> MGSHHHHHHSSGLVPRGSHMFKREEIIEMANKDFEKAWIETKDLIKAKKINESYPRIKPVFGKTHPVNDTIENLRQAYLRMGFEEYINPVIVDERDIYKQFGPEAMAVLDRCFYLAGLPRPDVGLSDEKISQIEKLGIKVSEHKESLQKILHGYKKGTLDGDDLVLEISNALEISSEMGLKILEDVFPEFKDLTAVSSKLTLRSHMTSGWFLTVSDLMNKKPLPFKLFSIDRCFRREQKEDKSHLMTYHSASCAIAGEGVDINDGKAIAEGLLSQFGFTNFKFIPDEKKSKYYTPETQTEVYAYHPKLKEWLEVATFGVYSPVALSKYGIDVPVMNLGLGVERLAMISGNFADVREMVYPQFYEHKLNDRNVASMVKLDKVPVMDEIYDLTKELIESCVKNKDLKSPCELAIEKTFSFGKTKKNVKINIFEKEEGKNLLGPSILNEIYVYDGNVIGIPESFDGVKEEFKDFLEKGKSEGVATGIRYIDALCFKITSKLEEAFVSNTTEFKVKVPIVRSLSDINLKIDDIALKQIMSKNKVIDVRGPVFLNVEVKIEXXXXXXXXXXXXXXXXXXXXXXXXXXXXXXXXXXXXXXXXXXXXXXXXXXXXXXXXXXXXXXXXXXXXXXXXXXXXXXXXXXXXXXXXXXXXXXXXXXXXXXXXXXXXX;> MGSHHHHHHSSGLVPRGSHMFKREEIIEMANKDFEKAWIETKDLIKAKKINESYPRIKPVFGKTHPVNDTIENLRQAYLRMGFEEYINPVIVDERDIYKQFGPEAMAVLDRCFYLAGLPRPDVGLSDEKISQIEKLGIKVSEHKESLQKILHGYKKGTLDGDDLVLEISNALEISSEMGLKILEDVFPEFKDLTAVSSKLTLRSHMTSGWFLTVSDLMNKKPLPFKLFSIDRCFRREQKEDKSHLMTYHSASCAIAGEGVDINDGKAIAEGLLSQFGFTNFKFIPDEKKSKYYTPETQTEVYAYHPKLKEWLEVATFGVYSPVALSKYGIDVPVMNLGLGVERLAMISGNFADVREMVYPQFYEHKLNDRNVASMVKLDKVPVMDEIYDLTKELIESCVKNKDLKSPCELAIEKTFSFGKTKKNVKINIFEKEEGKNLLGPSILNEIYVYDGNVIGIPE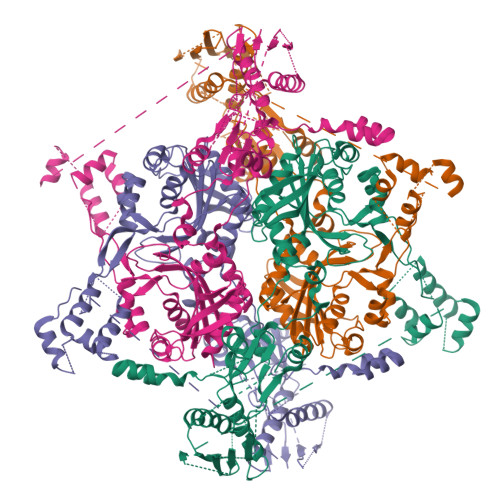SFDGVKEEFKDFLEKGKSEGVATGIRYIDALCFKITSKLEEAFVSNTTEFKVKVPIVRSLSDINLKIDDIALKQIMSKNKVIDVRGPVFLNVEVKIEXXXXXXXXXXXXXXXXXXXXXXXXXXXXXXXXXXXXXXXXXXXXXXXXXXXXXXXXXXXXXXXXXXXXXXXXXXXXXXXXXXXXXXXXXXXX;> MGSHHHHHHSSGLVPRGSHMFKREEIIEMANKDFEKAWIETKDLIKAKKINESYPRIKPVFGKTHPVNDTIENLRQAYLRMGFEEYINPVIVDERDIYKQFGPEAMAVLDRCFYLAGLPRPDVGLSDEKISQIEKLGIKVSEHKESLQKILHGYKKGTLDGDDLVLEISNALEISSEMGLKILEDVFPEFKDLTAVSSKLTLRSHMTSGWFLTVSDLMNKKPLPFKLFSIDRCFRREQKEDKSHLMTYHSASCAIAGEGVDINDGKAIAEGLLSQFGFTNFKFIPDEKKSKYYTPETQTEVYAYHPKLKEWLEVATFGVYSPVALSKYGIDVPVMNLGLGVERLAMISGNFADVREMVYPQFYEHKLNDRNVASMVKLDKVPVMDEIYDLTKELIESCVKNKDLKSPCELAIEKTFSFGKTKKNVKINIFEKEEGKNLLGPSILNEIYVYDGNVIGIPESFDGVKEEFKDFLEKGKSEGVATGIRYIDALCFKITSKLEEAFVSNTTEFKVKVPIVRSLSDINLKIDDIALKQIMSKNKVIDVRGPVFLNVEVKIEXXXXXXXXXXXXXXXXXXXXXXXXXXXXXXXXXXXXXXXXXXXXXXXXXXXXXXXXXXXXXXXXXEXXXXXXXXXXXXXXXXXXXXXXXXXXXXXXXXXXXXXXXXXXXXXXXXXXXXXXXXXXXXXXX>MTTVLPPLEDTDGLWAALTEAAASVEKLLATLPEHGARSSAERAEIAAAHDAARALRVRFLDTHADAVYDRLTDHRRVHLRLAELVEAAATAFPGLVPTQQQLAVERSLPQAAKEGHEIDQGIFLRAVLRSPLAGPHLLDAMLRPTPRALELLPEFVRTGEVEMEAVHLERRDGVARLTMCRDDRLNAEDGQQVDDMETAVDLALLDPGVRVGLLRGGVMSHPRYRGKRVFSAGINLKYLSQGGISLVDFLMRRELGYIHKLVRGVLTNDDRPGWWHSPRIEKPWVAAVDGFAIGGGAQLLLVFDRVLASSDAYFSLPAAKEGIIPGAANLRLGRFAGPRVSRQVILEGRRIWAKEPEARLLVDEVVEPDELDAAIE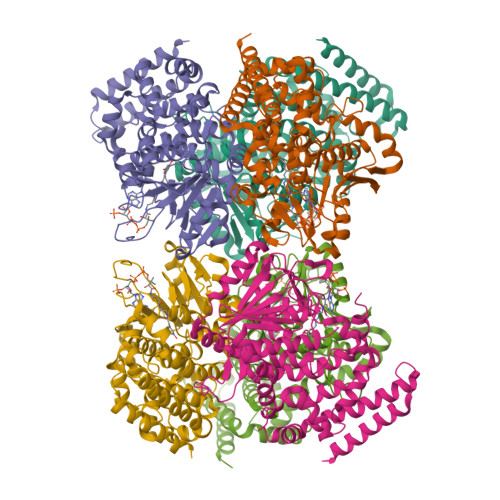RSLTRLDGDAVLANRRMLNLADESPDGFRAYMAEFALMQALRLYGHDTIDKVGRFGGRPPA[12x]>[2x]GPLGSRKGKDPKIEEFV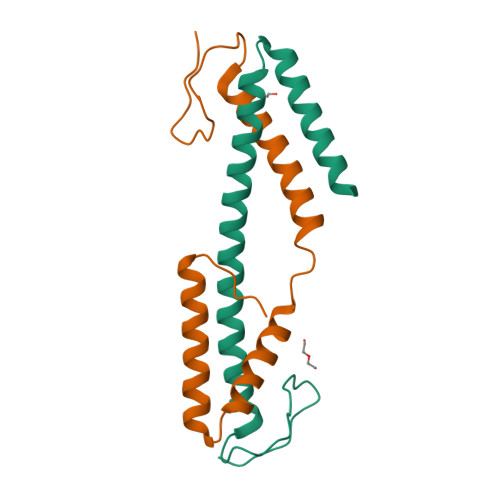PPDENCPLKEASSRRIPRLTVKAREHCLRLLEEALSSNRQSTRTADEADLRAKAVELEHETFRNAKVANLYKASVLKKVADIHRASKDGQPYDM Replication initiator proteins (Reps) from the HUH endonuclease family process specific single-stranded DNA sequences to initiate rolling-circle replication in viruses. Smacoviridae is a family of small CRESS-DNA (circular Rep-encoding single-stranded DNA) viruses. Named after a triad of residues, the HUH motif in the nickase domain is most often made up of two histidines separated by a bulky hydrophobic residue (U), but can also be histidine–U–glutamine. Recent comparisons of CRESS-DNA Rep-domain protein sequences show that smacovirus Rep domains are both the smallest in size and the most divergent in sequence of the CRESS-DNA viral Reps.

The structure of the human smacovirus 1 Rep domain was obtained at 1.33 Å resolution and represents an expansion of the HUH endonuclease superfamily, allowing greater diversity in bioconjugation-tag applications. To uncover structural differences compared with other ssDNA-bound HUH-tags, attempts to co-crystallize the ssDNA-bound protein were performed by mutating the catalytic tyrosine (Tyr81) to a phenylalanine. This allows the coordination of the ssDNA but not covalent linkage to the ssDNA. The crystal belonged to space group P211. There was one protein molecule in the asymmetric unit. Modeling of ssDNA in the electron density adjacent to the catalytic domains, HUQ and tyrosine motifs for the bound/coordinated structure was also unsuccessful. The resulting unbound structure consists of β1, α1, β2, β3, α2, β4 and α3 secondary structures, with the β-sheets in an antiparallel layout. The catalytically dead phenylalanine substituting for the reactive tyrosine residue resides within α3 and the coordinating histidine and glutamine residues reside within β3. HSV1 Rep is also structurally different from WDV Rep and PCV2 Rep in that α2 and α3 have shorter disordered loops connecting the α-helices to the β-sheets. Another difference among the families compared here is in the orientation of the HUH/Q and tyrosine residues in the catalytic motifs, but this could also be explained by the absence of the divalent metal ion that is required to prime the active site for nucleophilic attack on the DNA substrate.

> MTEPKWYDITVSKAKCPEEILRKWLDENGERYAYGRERGEDGYEHFQVRVVLRNPTSWETMREIWGNSGHCSPTSIRNFDFVLKEGDFVCSWIKVPD>MSTDKITFLLNWQPTPYHIPIFLAQTKGYFKEQGLDMAILEPTNPSDVTELIGSGKVDMGLKAMIHTLAAKARGFPVTSVASLLDEPFTGVLYLKGSGITEDFQSLKGKKIGYVGEFGKIQIDELTKHYGMKPEDYTAVRCGMNVAKYIIEGKIDAGIGIECMQQVELEEYLAKQGRPASDAKMLRIDKLACLGCCCFCTVLYICNDEFLKKNPEKVRKFLKAIKKATDYVLADPVKAWSGYIDFKPQLNNDLSYKQYQRCYAYFSSSLYNVHRDWKKVTGYGKRLAILPPDYVSNYTNEYLSWPEPEEVSDPLEATRLMAIHQEKCRQEGTFKRLALPAHHHHHH[8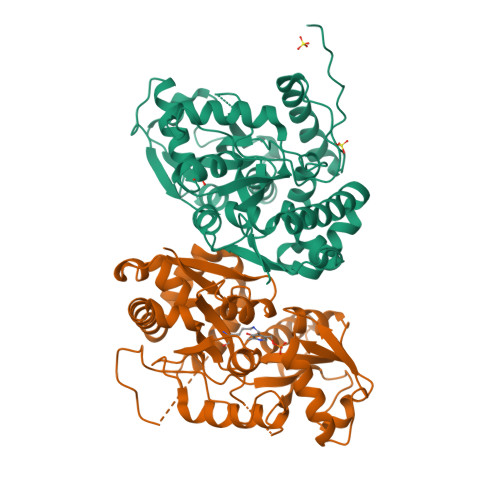x]>[2x]MEEPEEPADSGQSLVPVYIYSPEYVSMCDSLAKIPKRASMVHSLIEAYALHKQMRIVKPKVASMEEMATFHTDAYLQHLQKVSQEGDDDHPDSIEYGLGYDCPATEGIFDYAAAIGGATITAAQCLIDGMCKVAINWSGGWHHAKKDEASGFCYLNDAVLGILRLRRKFERILYVDLDLHHGDGVEDTFSFTSKVMTVSLHKFSPGFFPGTGDVSDVGLGKGRYYSVNVPIQDGIQDEKYYQIC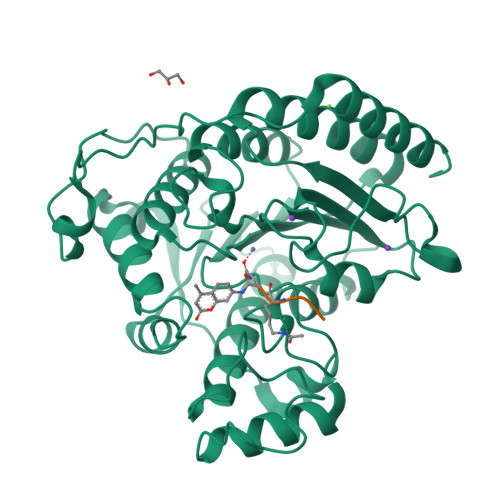ESVLKEVYQAFNPKAVVLQLGADTIAGDPMCSFNMTPVGIGKCLKYILQWQLATLILGGGGFNLANTARCWTYLTGVILGKTLSSEIPDHEFFTAYGPDYVLEITPSCRPDRNEPHRIQQILNYIKGNLKHVVIEGRGSHHHHHH;>[2x]XRHKK The LRR-RKs HAESA (greek: to adhere to) and HAESA-LIKE 2 (HSL2) redundantly control floral abscission. A receptor protein called HAESA is found on the surface of the cells that surround a future break point on the plant. When its time to shed an organ, a hormone called IDA instructs HAESA to trigger the shedding process. The peptide hormone IDA binds to the HAESA LRR ectodomain.

We next tested if HAESA binds other IDA peptide family members. IDL1, which can rescue IDA loss-of-function mutants when introduced in abscission zone cells, can also be sensed by HAESA, albeit with lower affinity. A 2.56 Å co-crystal structure with IDL1 reveals that different IDA family members use a common binding mode to interact with HAESA-type receptors. (E) Structural superposition of the active IDA (in bonds representation, in gray) and IDL1 peptide (in yellow) hormones bound to the HAESA ectodomain. Root mean square deviation (r.m.s.d.) is 1.0 Å comparing 100 corresponding atoms. Our comparative structural and biochemical analysis further suggests that IDLs share a common receptor binding mode, but may preferably bind to HAESA, HSL1 or HSL2 in different plant tissues and organs. Indeed, we find many of the residues contributing to the formation of the IDA binding surface in HAESA to be conserved in HSL2 and in other HAESA-type receptors in different plant species.

> GSSMGSLNQDATILRQAKLGLSDPAQSLSSWSDNNDVTPCKWLGVSCDATSNVVSVDLSSFMLVGPFPSILCHLPSLHSLSLYNNSINGSLSADDFDTCHNLISLDLSENLLVGSIPKSLPFNLPNLKFLEISGNNLSDTIPSSFGEFRKLESLNLAGNFLSGTIPASLGNVTTLKELKLAYNLFSPSQIPSQLGNLTELQVLWLAGCNLVGPIPPSLSRLTSLVNLDLTFNQLTGSIPSWITQLKTVEQIELFNNSFSGELPESMGNMTTLKRFDASMNKLTGKIPDNLNLLNLESLNLFENMLEGPLPESITRSKTLSELKLFNNRLTGVLPSQLGANSPLQYVDLSYNRFSGEIPANVCGEGKLEYLILIDNSFSGEISNNLGKCKSLTRVRLSNNKLSGQIPHGFWGLPRLSLLELSDNSFTGSIPKTIIGAKNLSNLRISKNRFSGSIPNEIGSLNGIIEISGAENDFSGEIPESLVKLKQLSRLDLSKNQLSGEIPRELRGWKNLNELNLANNHLSGEIPKEVGILPVLNYLDLSSNQFSGEIPLELQNLKLNVLNLSYNHLSGKIPPLYANKIYAHDFIGNPGLCVDLDGLCRKITRSKLEGSENLYFQ;> LVPPSGPSMRHN ISOQUINOLINE-5-SULFONIC 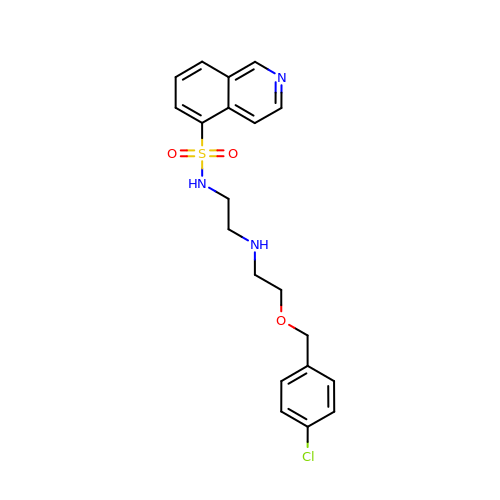ACID (2-(2-(4-CHLOROBENZYLOXY)ETHYLAMINO)ETHYL)AMIDE | C20 H22 Cl N3 O3 S | AUHWQSZMVMMRLM-UHFFFAOYSA-N>[2x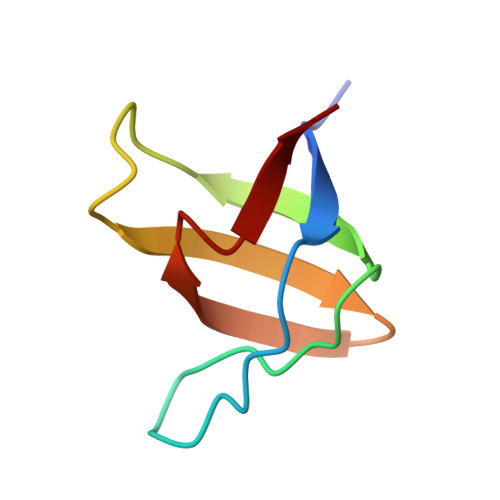]GAMATAVALYNFAGEQPGDLAFKKGDVITILKKSDSQNDWWTGRTNGKEGIFPANYVRVS> MADTQYILPNDIGVSSLDSREAFRLLSPTERLYAYHLSRAAWYGGLAVLLQTSPEAPYIYALLSRLFRAQDPDQLRQHALAEGLTEEEYQAFLVYAAGVYSNMGNYKSFGDTKFVPNLPKEKLERVILGSEAAQQHPEEVRGLWQTCGELMFSLEPRLRHLGLGKEGITTYFSGNCTMEDAKLAQDFLDSQNLSAYNTRLFKEVDGCGKPYYEVRLASVLGSEPSLDSEVTSKLKSYEFRGSPFQVTRGDYAPILQKVVEQLEKAKAYAANSHQGQMLAQYIESFTQGSIEAHKRGSRFWIQDKGPIVESYI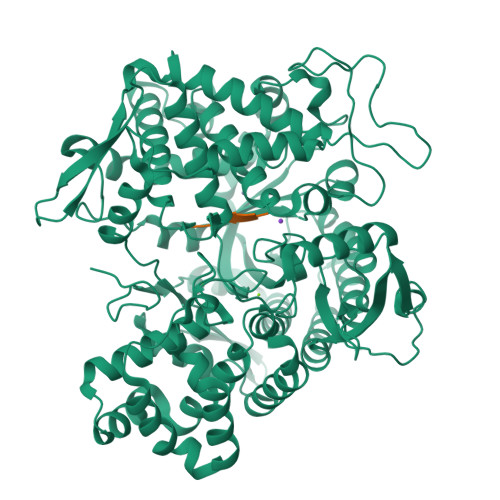GFIESYRDPFGSRGEFEGFVAVVNKAMSAKFERLVASAEQLLKELPWPPTFEKDKFLTPDFTSLDVLTFAGSGIPAGINIPNYDDLRQTEGFKNVSLGNVLAVAYATQREKLTFLEEDDKDLYILWKGPSFDVQVGLHALLGHGSGKLFVQDEKGAFNFDQETVINPETGEQIQSWYRCGETWDSKFSTIASSYEECRAESVGLYLSLHPQVLEIFGFEGADAEDVIYVNWLNMVRAGLLALEFYTPEAFNWRQAHMQARFVILRVLLEAGEGLVTITPTTGSDGRPDARVRLDRSKIRSVGKPALERFLRRLQVLKSTGDVAGGRALYEGYATVTDAPPESFLTLRDTVLLRKESRKLIVQPNTRLEGSDVQLLEYEASAAGLIRSFSERFPEDGPELEEILTQLATADARFW;> YGGFM> AQPDIKFASKEYGVTIGESRIIYPLDAAGVMVSVKNTQDYPVLIQSRIYDENKEKESEDPFVVTPPLFRLDAKQQNSLRIAQAGGVFPRDKESLKWLCVKGIPPKDEDIWVDDATN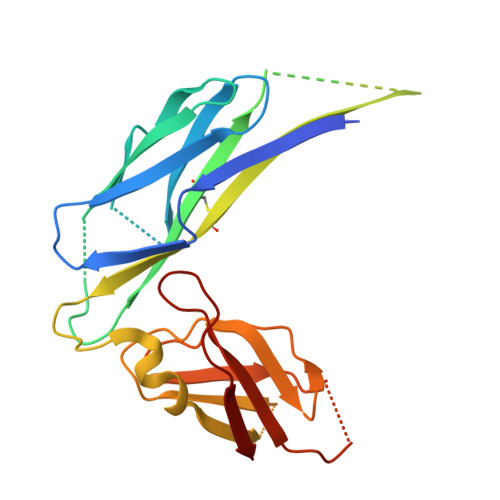KQKFNPDKDKDTNDVGVFVQFAINNCIKLLVRPNELKGTPIQFAENLSWKVDGGKLIAENPSPFYMNIGELTFGGKSIPSHYIPPKSTWAFDLPKGLAGARNVSWRIINDQGGLDRLYSKNVTL>MKYNNKFKSLALISVAAGLFFANPLQAATAISGTFFDKNNTSADMTVRAYSWYNLSMGYLGWTHHSNWGFVKLKKGKPVTIALTTEVSGLHPSITVWYRAGAKNPKTLPYMNGHAYKQFGDIYEPNAEATDAENNPVKVGNIIMKFITNGFDRDGMGDALPAEYDQSQLYRVMDGVPGKLAITFTPPENGWYQFVVGAINPDIDSTAYGSGPGSGAGPATAHTVHVEVSIP[6x]

A copper repressible protein, denoted CorA, was previously identified from a particulate fraction of M. album BG8 cells. In the present work, we show that CorA is non-covalently associated to the M. album BG8 outer membrane and exposed on the cellular surface, contrary to the previously assumed localization to the Gram-negative inner membranes. Furthermore, both endogenously- and recombinantly expressed CorA were purified to homogeneity, and inductively coupled plasma mass spectrometry (ICP-MS) analyses demonstrated that only endogenously expressed CorA binds copper, one atom per molecule. Moreover, our findings substantiate that CorA and its homologous proteins MopE and MEALZv2_1030034 play an active role in the copper handling/uptake, which again is necessary for providing copper to pMMO required for its methane monooxygenase enzymatic activity.

Native CorA crystals diffracted to a resolution of 1.6 Å. The asymmetric unit of the CorA crystals consists of six molecules forming two trimers. Consistent with the CD spectrum of rec-CorA, the structure contains mainly β-strands forming two β-sheets and random coils and very little helical content. CorA contains two metal ions, which by analogy to MopE* was interpreted as calcium and copper, and the latter confirmed by ICP-MS. The CorA copper-binding site closely resembles the mononuclear binding site present in MopE*, i.e. the copper atom is coordinated by two histidines, one water molecule, and the tryptophan metabolite kynurenine. The geometry is distorted tetrahedral with the copper ion almost at the base of the pyramid formed by residues Kyn62, H64 and H114 and the solvent molecule at the apical position displaying geometrical similarities to Type I (blue copper proteins) and CuB copper centres. The distance of the copper ion and the nitrogen atom of the kynurenine (2.9 Å) is considerably longer than what is usually considered a copper-nitrogen interaction. The kynurenine is, therefore, not a first-sphere ligand, but the ring amino group is close enough to be a second sphere copper ligand. The Ca2+ ion is bound in a somewhat distorted octahedral geometry with ligand-metal-ligand angles near 90 degrees and with metal-ligand bond distances of 2.3 to 2.4 Å. Our presumption is that the conserved Ca2+ binding site is important for the stabilization of the structures of these Cu(I) binding proteins.>GSSHHHHHHSSGLVPRGSMSTSWSDRLQNAADMPANMDKHALKKYRREAYHRVFVNRSLAMEKIKCFGFNMDYTLAVYKSPEYESLGFELTVERLVSIGYPQELLSFAYDSTFPT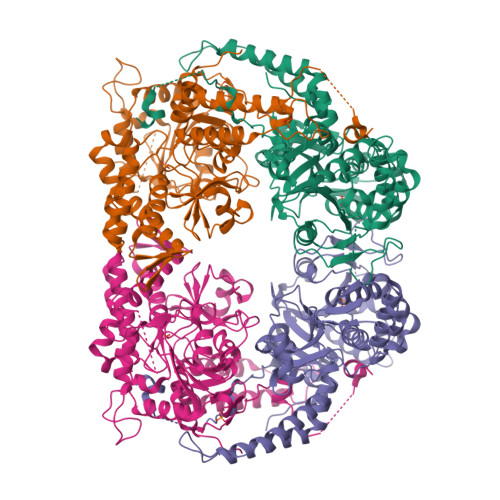RGLVFDTLYGNLLKVDAYGNLLVCAHGFNFIRGPETREQYPNKFIQRDDTERFYILNTLFNLPETYLLACLVDFFTNCPRYTSCETGFKDGDLFMSYRSMFQDVRDAVDWVHYKGSLKEKTVENLEKYVVKDGKLPLLLSRMKEVGKVFLATNSDYKYTDKIMTYLFDFPHGPKPGSSHRPWQSYFDLILVDARKPLFFGEGTVLRQVDTKTGKLKIGTYTGPLQHGIVYSGGSSDTICDLLGAKGKDILYIGDHIFGDILKSKKRQGWRTFLVIPELAQELHVWTDKSSLFEELQSLDIFLAELYKHLDSSSNERPDISSIQRRIKKVTHDMDMCYGMMGSLFRSGSRQTLFASQVMRYADLYAASFINLLYYPFSYLFRAAHVLMPHESTVEHTHVDINEMESPLATRNRTSVDFKDTDYKRHQ[2x]> ATGVRAVPGNENSLEIEELARFAVDEHNKKENALLEFVRVVKAKEQAMNTGFTLATMYYLTLEAKDGGKKKLYEAKVWVKNTQWHNAMTNFK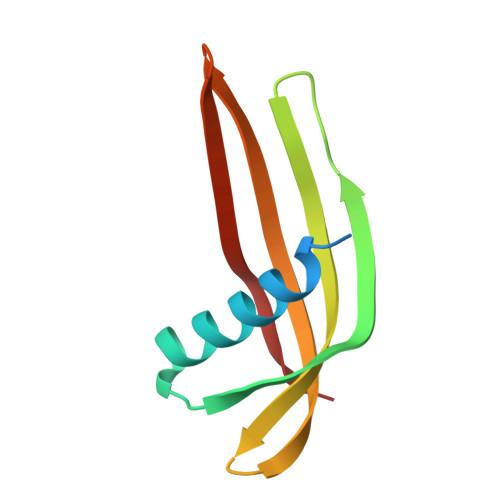ELQEFKPVG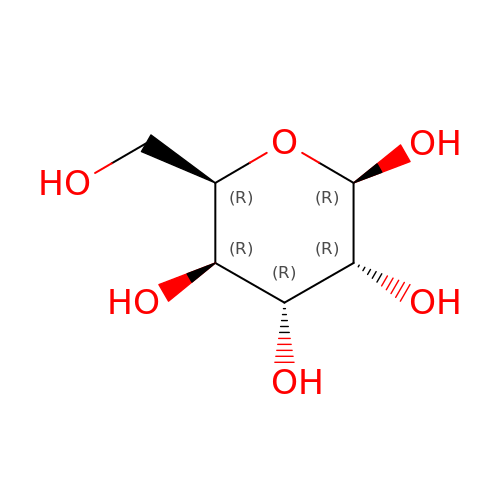beta-D-gulopyranose | C6 H12 O6 | WQZGKKKJIJFFOK-AIECOIEWSA-N>[2x]AMGIVIEKAADGYKLSIDGRETYIKGVGGTYRLDIAAQSGANAFRTWGGNV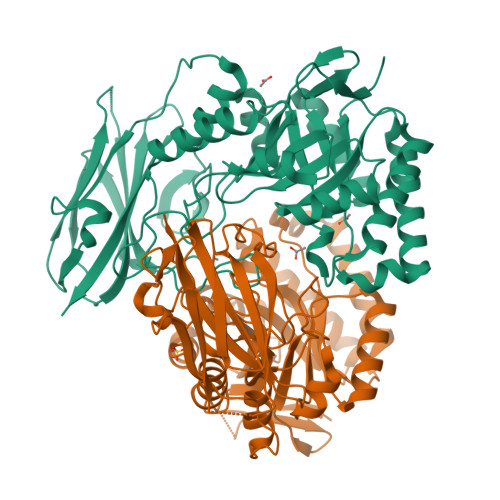EEIKKNLALASEHNMYVMQGIGMTKDSIRYYDDEYKNKMREEVRLLAETFKNDTSLLAWGIGNEIELGNANIAAAWNFVEELAQLIKSIDKRHLVSTVISYNPSALDSVAKYAPSLDYVGINVYGPMGEVQAVVDRSDYKGAFMITEWGPTGWWETASTEWKAPIEQTSEEKRQVYEERYTQYISANTRCLGSFVFLWGQKEERTPTWFSMFVEDKVDSLPLKGEKTPMVEAMQRVWTGKELDETAPIVRGMTIDGKSAIDNVRIKAGTLFKAEVSVTDKENDSLAYVWEVLKEATVLGFGGSYEPRPERMGDVAVSDKNVYETMIKVPGEYRLYVYVLDNTGFVSTANIPFQVID> GSHMQPEQKASNLIGTYRHVDRATGQVLTCDKCPAGTYVSEHCTNTSLRVCSSCPVGTFTRHENGIEKCHDCSQPCPWPMIEKLPCAALTDRECTCPPGMFQSNATCAPHTVCPVGWGVRKKGTETEDVRCKQCARGTFSDVPSSVMKCKAYTDCLSQNLVVIKPG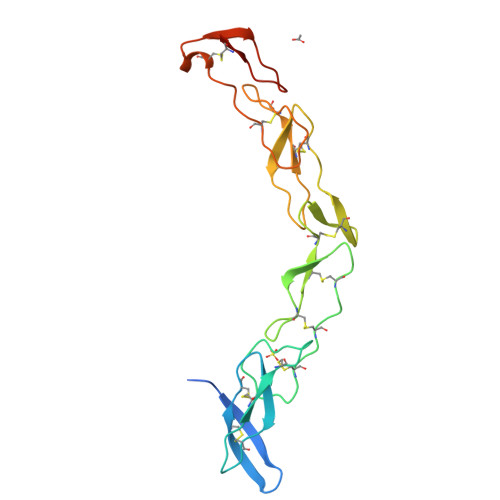TKETDNVCGTLPSFS2-[[(3~{S})-2,6-bis(oxidanylidene)piperidin-3-yl]carbamoyl]benzoic acid | C13 H12 N2 O5 | 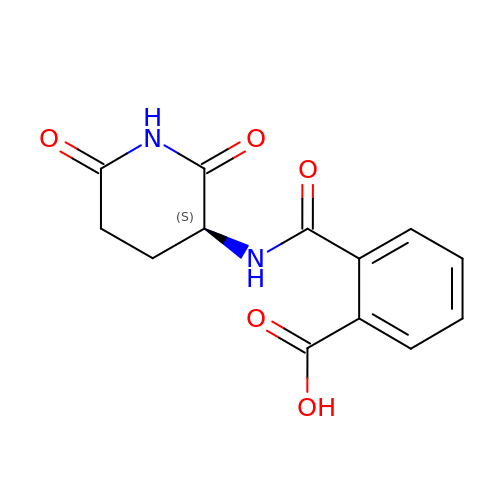QTUSGYNZYGYXIN-VIFPVBQESA-N>MSLSDESFEFDVSVIGLGAMGTIMAQVLLKQGKRVAIWNRSPGKAAALVAAGAHLCESVKAALSASPATIFVLLDNHATHEVLGMPGVARALAHRTIVDYTTNAQDEGLALQGLVNQAG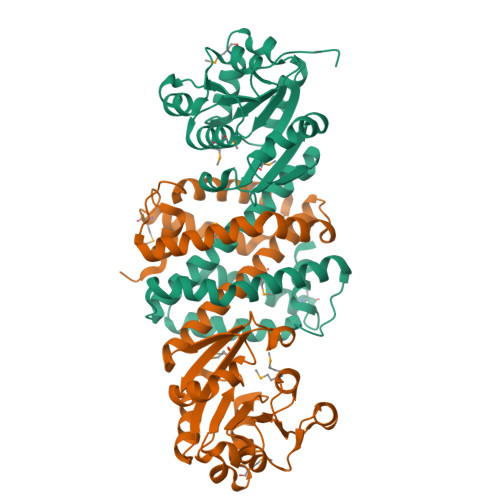GHYVKGMIVAYPRNVGHRESHSIHTGDREAFEQHRALLEGLAGHTVFLPWDEALAFATVLHAHAFAAMVTFFEAVGAGDRFGLPVSKTARLLLETSRFFVADALEEAVRRLETQDFKGDQARLDVHADAFAHIAQSLHAQGVWTPVFDAVCQVVQRAAAMGYGDQDIAATTKSFAREQEEGHHHHHH[2x]> MHHGFTT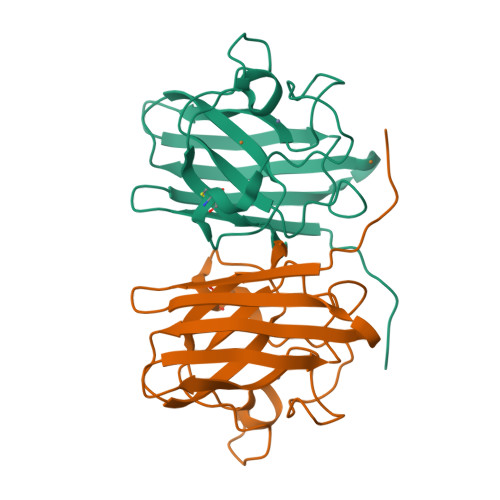PSRAIAVLSTETIRGNITFTQVQDGKVHVQGGITGLPPGEYGFHVHEKGDLSGGCLSTGSHFNPEHKDHGHPNDVNRHVGDLGNVVFDENHYSRIDLVDDQISLSGPHGIIGRAVVLHEKADDYGKSDHPDSRKTGNAGGRVACGVIGIL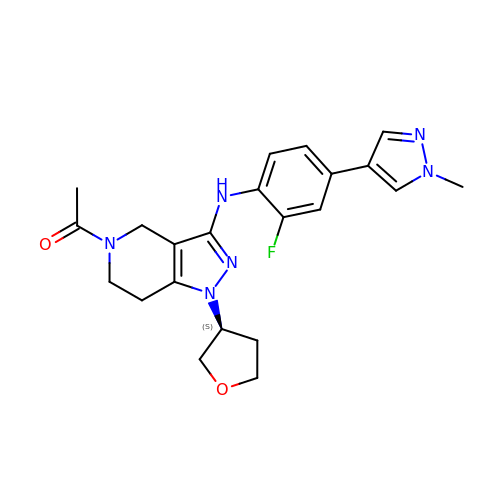1-[3-[[2-fluoranyl-4-(1-methylpyrazol-4-yl)phenyl]amino]-1-[(3~{S})-oxolan-3-yl]-6,7-dihydro-4~{H}-pyrazolo[4,3-c]pyridin-5-yl]ethanone | C22 H25 F N6 O2 | NKOJNOBJGYTLLZ-KRWDZBQOSA-N Here we report the biochemical characterization of the AA12 enzyme encoded by the genome of the ascomycete Trichoderma reesei (TrAA12). The three-dimensional structure of TrAA12 reveals important similarities with bacterial soluble glucose dehydrogenases (sGDH). TrAA12 preferentially oxidizes l-fucose, and weak activity was measured against d-arabinose (11.6% relative activity), d-galactose (5.7%), l-arabinose (2.8%), and d-lyxose (2.2%). Based on these results, the AA12 family of enzymes is likely to have a catalytic mechanism close to that of bacterial sGDH.

The polypeptide chain observable in the crystal structure of TrAA12 covers amino acids Gln24 to Asn435. This domain folds as a 6-blade β-propeller. The three structures superimposed very well, and no major differences in the main chains were observed. All the structures solved present a constitutive calcium. This calcium stabilizes a long loop which joins sheets C and D of the fourth blade. The calcium ion presents a typical octahedral coordination. Three amino acids are directly involved in the coordination: Glu259 and Gln301 with their side chains and Tyr276 by the main chain. Three water molecules complete the coordination, stabilized mainly by the side chains of Glu238 and Asn26. Of the seven predicted N-glycosylation sites, five are visible in the density maps on Asn94, Asn147, Asn184, Asn306, and Asn341. The two longer N-glycans, on Asn94 and Asn306, come close to the symmetric molecule and participate in crystal packing.

> TTNNLQVTYPAPVAADGWEYRLISTGLTAPRSIVFDSTGGLLVLDAGVGVRRLTLQDNGGTCLSVTANATLIADTALNHGLAISADGGTIYASTVNDVYAYTYNEQTNTVDPTTRRTVVTNMTNTDHVTRTLLLSSRLPNELLVSRGSAANEDPQARNVTSGHSQIRAYDISTLAATDPPFDFVAGTLIGWGLRDSVGVGENPTNGGIWSVENSVDDLTREGVDVHQDNPGEELNFHGILGNTANQGGNYGYPDCYALWSTAGFPDLGALEVGDQFASDNATAGVTDATCNTNFVDPRLVFQAHVSPLDIKFNTNGTTAYITFHGSTDRTTPVGYSIVSVAFGLNGQPTSPMDSTTAANNILTSPDLTQCPDDCFTPVGLTFDTIGRLFFSSDSTGEIFVLQQS>MNKTELINAVAETSGLSKKDATKAVDAVFDSITEALRKGDKVQLIGFGNFEVRERAARKGRNPQTGEEMEIPASKVPAFKPGK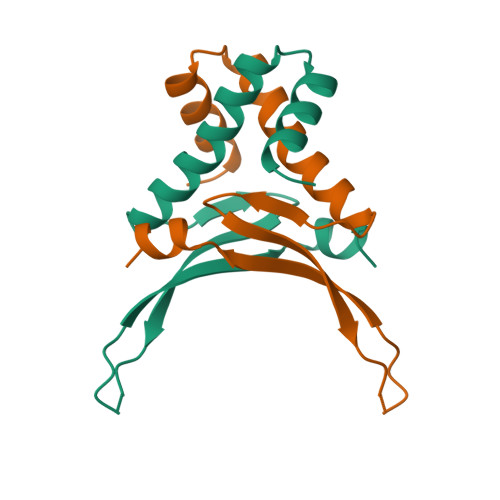ALKDAVK[3x]> LPTLGPGWQRQNPDPPVSRTRSLLLDAASGQLRLEDGFHPDAVAWANLTNAIRETGWAYLDLSTNGRYNDSLQAYAAGVVEASVSEELIYMHWMNTVVNYCGPFEYEVGYCEKLKNFLEANLEWMQREMELNPDSPYWHQVRLTLLQLKGLEDSYEGRLTFPTGRFTIKPLGFLLLQISGDL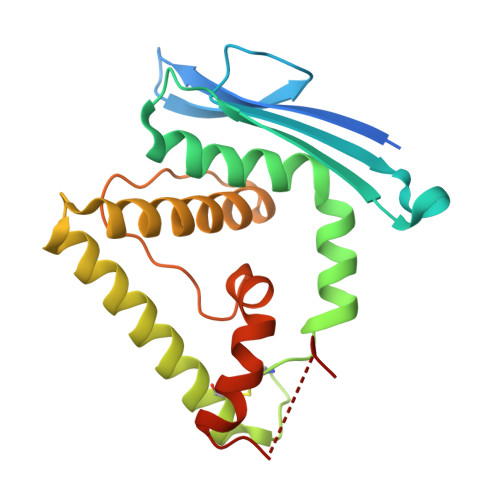EDLEPALNKTNTKPSLGSGS>MNTINIAKNDFSDIELAAIPFNTLADHYGERLAREQLALEHESYEMGEARFRKMFERQLKAGEVADNAAAKPLITTLLPKMIARINDWFEEVKAKRGKRPTAFQFLQEIKPEAVAYITIKTTLACLTSADNTTVQAVASAIGRAIEDEARFGRIRDLEAKHFKKNVEEQLNKRVGHVYKKAFMQVVEADMLSKGLLGGEAWSSWHKEDSIHVGVRCIEMLIESTGMVSLHRQNAGVVGQDSETIELAPEYAEAIATRAGALAGISPMFQPCVVPPKPWTGITGGGYWANGRRPLALVRTHSKKALMRYEDVYMPEVYKAINIAQNTAWKINKKVLAVANVITKWKHCPVEDIPAIEREELPMKPEDIDMNPEALTAWKRAAAAVYRKDKARKSRRISLEFMLEQANKFANHKAIWFPYNMDWRGRVYAVSMFNPQGNDMTKGLLTLAKGKPIGKEGYYWLKIHGANCAGVDKVPFPERIKFIEENHENIMACAKSPLENTWWAEQDSPFCFLAFCFEYAGVQHHGLSYNCSLPLAFDGSCSGIQHFSAMLRDEVGGRAVNLLPSETVQDIYGIVAKKVNEILQADAINGTDNEVVTVTDENTGEISEKVKLGTKALAGQWLAYGVTRSVTKRSVMTLAYGSKEFGFRQQVLEDTIQPAIDSGKGLMFTQPNQAAGYMAKLIWESVSVTVVAAVEAMNWLKSAAKLLAAEVKDKKTGEILRKRCAVHWVTPDGFPVWQEYKKPIQTRLNLMFLGQFRLQPTINTNKDSEIDAHKQESGIAPNFVHSQDG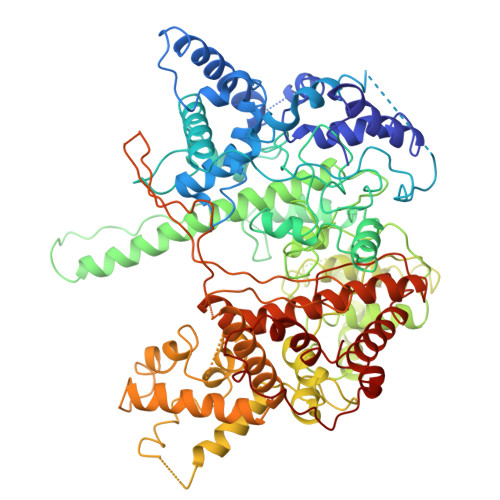SHLRKTVVWAHEKYGIESFALIHDSFGTIPADAANLFKAVRETMVDTYESCDVLADFYDQFADQLHESQLDKMPALPAKGNLNLRDILESDFAFA[3x]ACARBOSE DERIVED HEPTASACCHARIDE | C44 H74 N2 O30 | 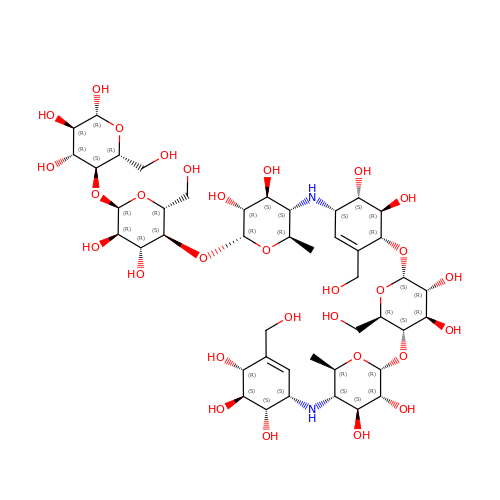DPMZCIRBUMLZIZ-BKAOIQCJSA-N> FACKTANGTAIPIGGGSANVYVNLAPAVNVGQNLVVDLSTQIFCHNDYPETITDYVTLQRGSAYGGVLSSFSGTVKYNGSSYPFPTTSETPRVVYNSRTDKPWPVALYLTPVSSAGGVAIKAGSLIAVLILRQTNNYNSDDFQFVWNIYANNDVVVPTGGCDVSARDVTVTLPDYPGSVPIPLTVYCAKSQNLGYYLSGTTADAGNSIFTNTASFSPAQGVGVQLTRNGTIIPANNTVSLGAVGTSAVSL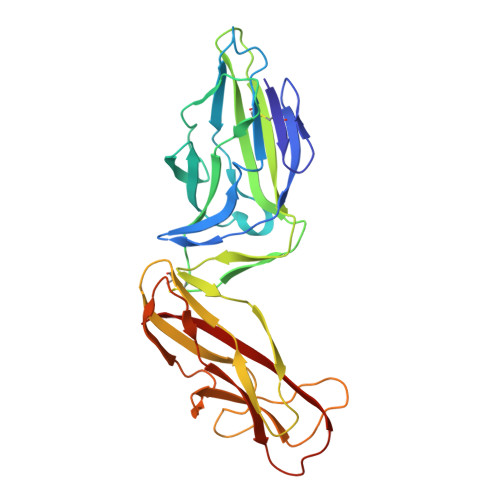GLTANYARTGGQVTAGNVQSIIGVTFVYQ>MGLAVFLPPYPFRGLKAPYLWMFYKYLHCATDSILFITGEDYLSVTDDEAQRARWEFDPASMASLGYELPNAQSMACHEYLTLDNAFYETLLSRHHHDPIKSFSAFLTERIPDLETELHALLDSKKGIIDQIDTFISICNCPSLEHVARTLGKEVMHIEIGPLRAPMYRNTAYLDFAGVNGGTEASARYEKCQAEFDIKASLGDLHNYFLEVLPPAEAATHSAAGVVLQVEDNSNLIAYNHDFTNISLLSYVRQRYEKEDILVRAHPGSLFRLRDDVFTIDDSANSLAFINQCNEVFTINSSVGLEAILTGKKTTVLGDCSYAFINELAGASATVNAAAFYLFSYLVPFDLVFNQEYLKFRLGHPEEREIVGKHIEFYSADMPGSLSQAAHSLSSLINEAISLEHHHHHH[2x]

WbbB, a lipopolysaccharide O-antigen synthesis enzyme from Raoultella terrigena, contains an N-terminal glycosyltransferase domain with a highly modified architecture that adds a terminal β-Kdo (3-deoxy-d-manno-oct-2-ulosonic acid) residue to the O-antigen saccharide, with retention of stereochemistry. WbbB’s two C-terminal GT domains produce a polymer with a [4)-α-Rhap-(1→3)-β-GlcpNAc-(1→] repeat unit, while the N-terminal domain of the protein contains a GT99 retaining β-Kdo transferase, referred to here as WbbBGT99. Kdo addition blocks further polymerization while creating the epitope recognized by the carbohydrate-binding module of the cognate ABC transporter, allowing export prior to ligation to lipid A-core in the periplasm. The evidence presented above strongly argues that WbbBGT99 is a retaining glycosyltransferase that uses a double-displacement mechanism analogous to that used by retaining glycoside hydrolases.

We next determined the structure of both the WbbBGT99-D232N (at 1.9 Å) and WbbBGT99-D232C (at 1.95 Å) variants as Kdo adducts. The WbbBGT99-D232N variant crystal was grown as a CMP complex, then soaked with a CMP-β-Kdo-generating reaction mix for five minutes before freezing. For both variants, clear additional density was present that could readily be modelled as an α-Kdo with an unambiguous linkage to the anomeric carbon. After refinement, in the WbbBGT99-Asn232–Kdo structure, Kdo has a 0.7 occupancy, with ADPs similar to those of surrounding side chains (suggesting around 70% conversion to the adduct), while the resulting electron density clearly defines the positions of all atoms. Significantly more adduct is apparent in the structure than was observed by LC/MS, supporting the idea that this adduct forms quickly, and then undergoes gradual hydrolysis with a half-life on an hour-time scale. The Asn- and Cys- Kdo adduct structures refine with α-Kdo in a very similar position, with only small shifts (0.29 Å r.m.s.d. for Kdo compared to 0.24 Å for the protein), with the largest shifts in the anomeric carbon (0.6 Å) and carboxylate residue. The most striking feature of the adduct structure is the dramatic reorganization of the Kdo group relative to the CMP-β-Kdo complex, with the C1 carboxylate moved furthest away from the leaving group phosphate, the exocyclic O8 group closest, and the anomeric carbon shifted 6.1 Å from the leaving group phosphate oxygen. The carboxylate group interacts with Arg12, as well as Ser233; in the WbbBGT99-D232N–Kdo structure, the hydrogen bond is to Ser233 N, while a ~30° rotation of the carboxylate group reorients this oxygen in the WbbBGT99-D232C–Kdo structure to instead hydrogen bond with the Ser233 Oγ. The Kdo O4 forms hydrogen bonds with Glu158 and Asn179 (as well as a structured water); O6 forms a pair of hydrogen bonds with Arg163 as well as the CMP phosphate oxygen.> MLGAVEGPRWKQAEDIRDIYDFRDVLGTGAFSEVILAEDKRTQKLVAIK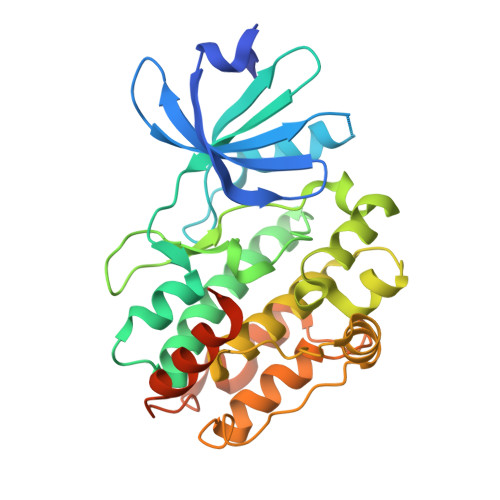CIAKEALEGKEGSMENEIAVLHKIKHPNIVALDDIYESGGHLYLIMQLVSGGELFDRIVEKGFYTERDASRLIFQVLDAVKYLHDLGIVHRDLKPENLLYYSLDEDSKIMISDFGLSKMEDPGSVLSTACGTPGYVAPEVLAQKPYSKAVDCWSIGVIAYILLCGYPPFYDENDAKLFEQILKAEYEFDSPYWDDISDSAKDFIRHLMEKDPEKRFTCEQALQHPWIAGDTALDKNIHQSVSEQIKKNFAKSKWKQAFNATAVVRHMRKLQ>[4x]MSKTIIKNIGKIVSGDIKSPVLQADT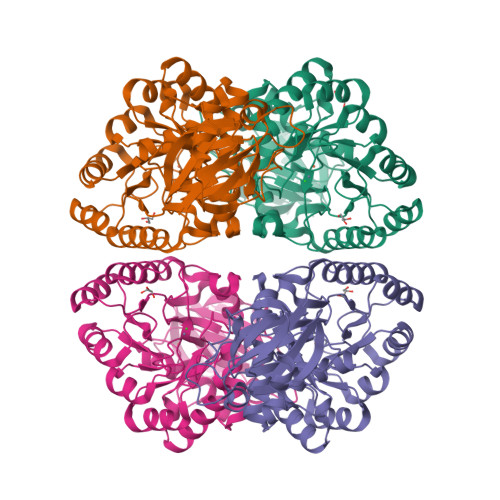IVVEDGLIAAIGGEELMKDAGDATIIDAAGSTVTPGLLDTHVHVSGGDYAPRQKTMDFISSALHGGVTTMISAGSPHFPGRPKDAAGTKALAITLSKSYYNARPAGVKVHGGAVILEKGLTEEDFIEMKKEGVWIVGEVGLGTIKNPEDAAPMVEWAHKHGFKVQMHTGGTSIPGSSTVTADDVIKTKPDVVSHINGGPTAISVQEVDRIMDETDFAMEIVQCGNPKIADYVARRAAEKGQLGRVIFGNDAPSGTGLIPLGILRNMCQIASMSDIDPEVAVCMATGNSTAVYGLNTGVIAPGKEADLIIMDTPLGSVAEDAMGAIAAGDIPGISVVLIDGEAVVTKSRNTPPAKRAAKIL>MGSDKIHHHHHHMTEIATIEKPAQHGATTRLIDIVFPG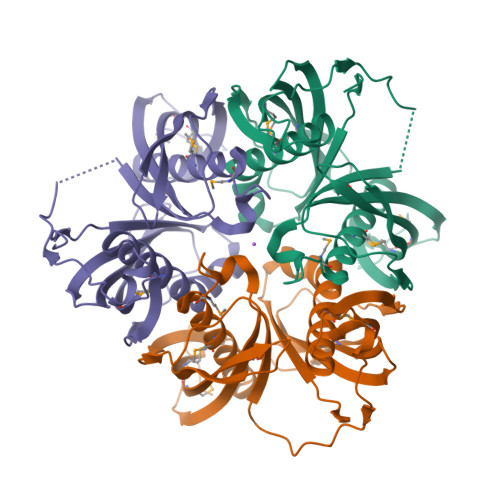DTNHHGTLFGGTGLALMDRVAFIAATRFGRTPFVTASCERIDFRQPARIGHIVEFTARPVKAGRRSLTVEVEMVAETIIGRQQHTCTRGIFHMVAIPEGEDAASYVLPELLTEETPDPSDAVTMVEIVFPDQANSAGRMFGGEAIAYMTKAAFVAASRYCGKLVVLASSERIDFARAIEIGEIVEAQAHVERVGRSSMSIQTKLWSENLLTGERHITATGHFTMVAVDKDHRPATIRDPAEAFSLEKGGA[3x]S-[2-[3-[[(2R)-3,3-dimethyl-2-oxidanyl-4-phosphonooxy-butanoyl]amino]propanoylamino]ethyl] 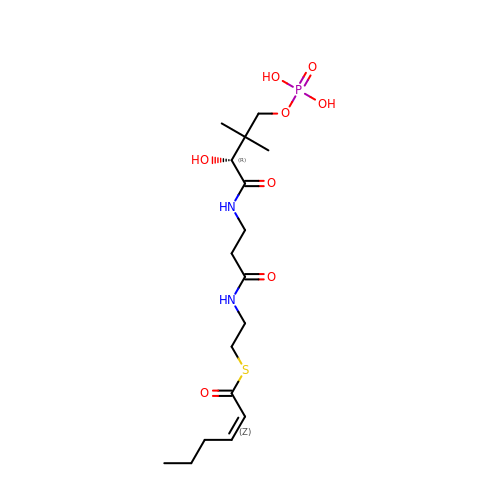(Z)-hex-2-enethioate | C17 H31 N2 O8 P S | IGFUSVMDVYHKKE-XHPSBEMXSA-N>GPGSEENEDSDPLPDNWE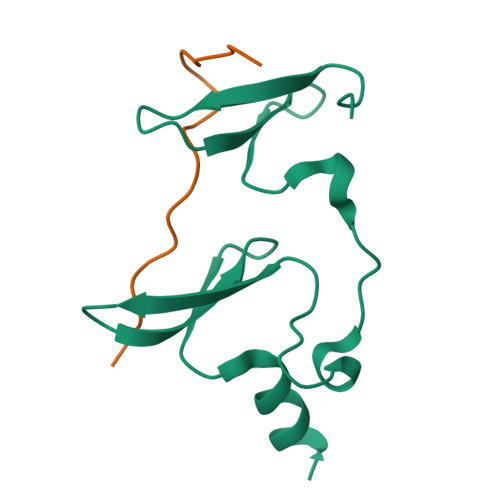MAYTEKGEVYFIDHNTKTTSWLDPRLAKKAKPPEECKENELPYGWEKIDDPIYGTYYVDHINRRTQFENPVLEAKRKLQQHN[2x];>GPGSDRPPPYVAPPSYEGPHRTLG[2x]Complementary DNA analyses revealed 22 distinct but similar peptides encoded by milk genes with homology to the lipocalin family of lipid-binding proteins, which are referred to as lipocalin-like milk proteins or Lili-Mip in this article. The data revealed glycosylated proteins that adopt a lipocalin fold, bind lipids and organize to form a tightly packed crystalline lattice. Lili-Mip serves as a complete nutrient by providing all of the essential amino acids, carbohydrates from the attached glycans, and lipids through chaperoning linoleic and oleic acids. After ingestion by the embryos, its increasing concentration in the midgut facilitates the crystallization of Lili-Mip.

Surprisingly, these protein crystals diffracted to 1.2 Å resolution and we report the first structure of a naturally occurring and chemically unaltered, heterogeneous protein crystal grown in vivo at atomic resolution. A complete native data set was collected from a single crystal that diffracted to 1.2 Å resolution. c electron-density maps of the 1.2 Å resolution structure revealed densities for glycosylation at Asn35, Asn66, Asn79 and Asn145. At positions 35 and 79, one β-mannose (BMA) and two NAGs were identified. The NAG molecules are linked to one another and to the mannose molecules via β(1→4) glycosidic bond linkages. The crystallographic data concurred with the MS data for the presence of four N-linked glycosylation sites. Mass analysis of Lili-Mip crystals shows the presence of linoleic and oleic acids. In the crystal structure, we observed a long fatty-acid chain in the barrel that we surmise to be either linoleic acid or oleic acid. Residues Val51, Val65, Thr81, Ser86, Phe100 and Leu113 line the binding pocket and show multiple conformations, suggesting that both oleic acid-bound and linoleic acid-bound proteins co-exist in the crystal. We can conclude from these observations that the monomer obtained in each asymmetric unit is a space average from all of the sequences, i.e. the crystal is made from packing of proteins with multiple sequences.

> IAAILVANAKEPCPPENLQLTPRALVGKWYLRTTSPDIFKQVSNITEFYSAHGNDYYGTVTDYSPEYGLEAHRVNLTVSGRTLKFYMNDTHEYDSKYEILAVDKDYFIFYGHPPAAPSGLALIHYRQSCPKEDVIKRVKKALKNVCLDYKYFGNDTSVPCHYVE>GSSGSSGMQIGKIIKVSGPLVMAENMSEASIQDMCLVGDLGVIGEIIEMRQDVASIQVYEETSGIGPGEPVRSTGEALSVELGPGIISQMFDGIQRPLDTFMEVTQSNFLGRGVQLPALDHEKQWWFE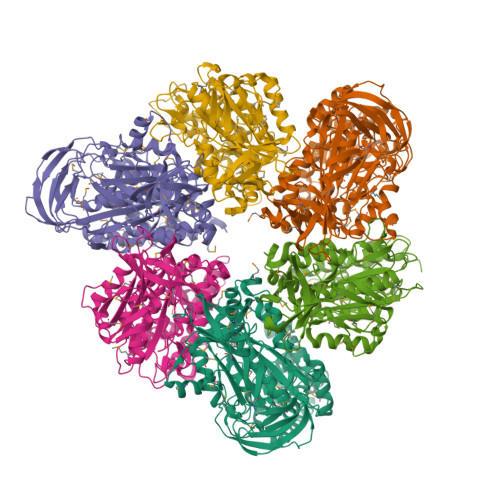ATIEEGTEVSAGDIIGYVDETKIIQHKIMVPNGIKGTVQKIESGSFTIDDPICVIETEQGLKELTMMQKWPVRRGRPIKQKLNPDVPMITGQRVIDTFFPVTKGGAAAVPGPFGAGKTVVQHQIAKWSDVDLVVYVGCGERGNEMTDVVNEFPELIDPNTGESLMERTVLIANTSNMPVAAREASIYTGITIAEYFRDMGYDVAIMADSTSRWAEALREMSGRLEEMPGDEGYPAYLGSRLAEYYERSGRVIALGSDQREGSITAISAVSPSGGDISEPVTQNTLRVVKVFWGLDSSLAQKRHFPSINWIQSYSLYSTEVGRYMDQILQQDWSDMVTEGMRILQEEEQLNEIVRLVGIDSLSDNDRLTLEVAKSIREDYLQQNAFDDVDTFTSREKQFNMLKVILTFGKEARKALSLGAYFNEIMEGTVAVRERISRSKYIPEEELAKISSINEEIKETIQLIVSEGGMTDD[3x];>[3x]GSSGSSGMIKEYRTIKEVVGPLMAVEKVSGVKYEELIEVRMQNGEIRRGQVLEVQEDKAMVQIFEGTSGINLKNSSVRFLGHPLQLGVSEDMIGRVFDGLGRPKDNGPEILPEKYLDINGEVINPIARDYPDEFIQTGISAIDHLNTLVRGQKLPVFSGSGLPHKELAAQIARQATVLDSSDDFAVVFAAIGITFEEAEFFMEDFRQTGAIDRSVMFMNLANDPAIERIATPRMALTAAEYLAYEKGMHVLVIMTDMTNYAEALREISAARREVPGRRGYPGYLYTNLATLFERAGRIRGLKGSVTQIPILTMPEDDKTHPIPDLTGYITEGQIILTRELYKSGIQPPIDVLPSLSRLKDKGTGAGKTREDHAATMNQLFAAYAQGKQAKELAVVLGESALSDIDKIYAKFAERFENEYVNQGFYTNRTITETLDLGWELLAMLPRTELKRIKDDLLDKYLPEGK> LEED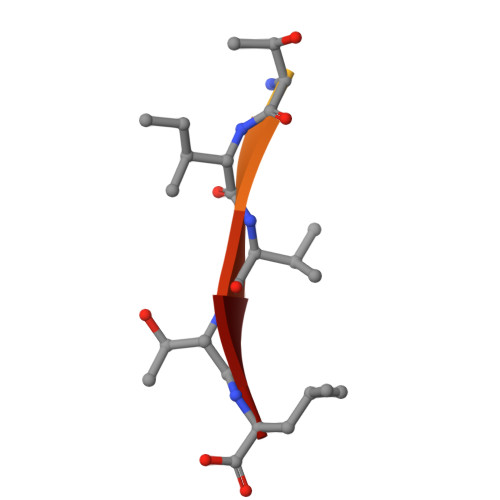GTIITL>MAKKDEVGGRVLQDVFLDWAKKYGPVVRVNVFHKTSVIVTSPESVKKFLMSTKYNKDSKMYRALQTVFGERLFGQGLVSECNYERWHKQRRVIDLAFSRSSLVSLMETFNEKAEQLVEILEAKADGQTPVSMQDMLTYTAMDILAKAAFGMETSMLLGAQKPLSQAVKLMLEGITASRNTLAKFLPGKRKQLREVRESIRFLRQVGRDWVQRRREALKRGEEVPADILTQILKAEEGAQDDEGLLDNFVTFFIAGHETSANHLAFTVMELSRQPEIVARLQAEVDEVIGSKRYLDFEDLGRLQYLSQVLKESLRLYPPAWGTFRLLEEETLIDGVRVPGNTPLLFSTYVMGRMDTYFEDPLTFNPDRFGPGAPKPRFTYFPFSLGHRSCIGQQFAQMEVKVVMAKLLQRLEFRLVPGQRFGLQEQATLKPLDPVLCTLRPRGWQP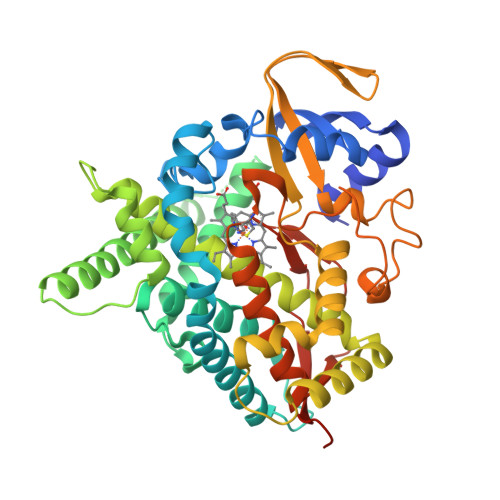APPPPPCHHHH[2x]>MCMAKVVLTKADGGRVEIGDV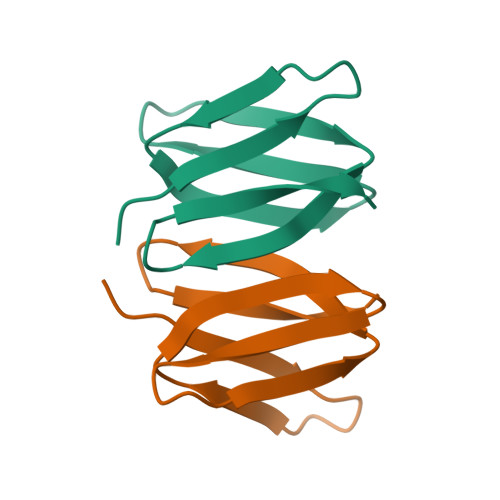LEVRAEGGAVRVTTLFDEEHAFPGLAIGRVDLRSGVISLIEEQNR[6x]>QVVAAIRHITTGTYIARIREEYQQTEVKPELQPMKEALARMT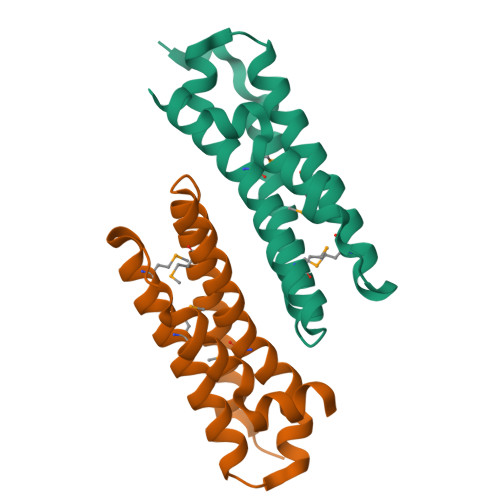DRAEALIAFVTEQKDQELLDFQARRLVEMTAHAVFGHLLMLAANDDDSFRQSAEVYLRYGQAEQEKIDSYVRAFRPEELTFYSRCSRPE[2x]~{N}-(4-hydroxyphenyl)-4-methyl-piperidine-1-carboxamide 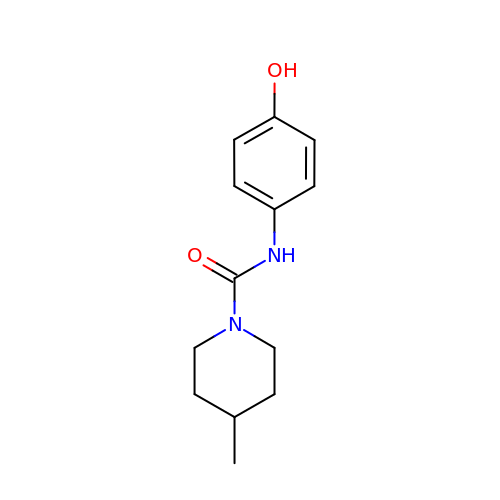| C13 H18 N2 O2 | UZAHGCAHTQUCTG-UHFFFAOYSA-N In the present work, we present the purification and biochemical characterization of a mJRL from the stem of Ananas comosus (AcmJRL). Size-exclusion chromatography clearly showed that AcmJRL is a homodimeric lectin in solution. AcmJRL adopt the expected β-prism fold with the three characteristic Greek key four-stranded β-sheets (β1–2 + β11–12, β3–6 and β7–10) and all the connecting loops well defined in the electron density. The structure of AcmJRL is the second structure of a mJRL reported with two carbohydrate-binding sites per monomer after BanLec.

Two structures of AcmJRL in complex with D-mannose (AcmJRL:Man) and methyl-α-D-mannopyranoside (AcmJRL:MeαMan) were obtained at 2.75 Å and 1.9 Å respectively. In both cases, the asymmetric unit contains two molecules. They form the side-by-side dimer in AcmJRL:Man and the tail-to-tail dimer in AcmJRL:MeαMan. In the AcmJRL:Man complex, four extra densities were interpreted as D-mannose molecules, two at the same positions in each monomer. One interacts with Greek key 1 (site 1) and one with Greek key 2 (site 2). In site 1, D-mannose oxygens are within hydrogen binding distance of the two carboxyl oxygens of Asp136 (O4 and O6), the hydroxyl of Ser133 (O5), and the backbone nitrogen of Gly15 (O3), Ser133 (O5) and Leu134 (O6). In site 2, the binding mode is similar to site 1, and the D-mannose oxygens interact similarly with the two carboxyl oxygens of Asp39 (O4 and O6) and the backbone nitrogen of Gly62 (O3), His36 (O5) and Ala37 (O6). In the AcmJRL:Man and AcmJRL:MeαMan complexes, the distance between the oxygen O4 of the ligand and Cβ of Glu14 is only 3.4 Å. This represents an unfavorable contact that could be responsible for the slightly lower affinity of AcmJRL for D-mannose and mannose-containing oligosaccharides. In the complex structures of AcmJRL, the distance between the O1 oxygens of the two binding sites is about 14 Å, making it impossible for mannopentaose to be bound in both site in the conformations observed in the AcmJRL:Man complex structures.

>SGLVKLGLWGGNEGTLQDIDGHPTRLTKIVIRSAHAIDALQFDYVEDGKTFAAGQWGGNGGKSDTIEFQPGEYLIAIKGTTGALGAVTNLVRSLTFISNMRTYGPFGLEHGTPFSVPVASGRIVAFYGRFGSLVDAFGIYLMPY[2x]>GPAASAGRIERRRARAAVAGRDATGRFTAGQPRRVELDADATSGAFYARYRDGYVSGEPWPGAGPPPPGRVLYGGLGDSRPGLWGAPEAEEARRRFEASGAPAAVWAPELGDAAQQYALITRLLYTPDAEAMGWLQNPRVVPGDVALDQACFRISGAARNSSSFITGSVARAVPHLGYAMAAGRFGWGLAHAAAAVAMSRRYDRAQKGFLLTSLRRAYAPLLARENAALTG[4x];> FTAG

The IE gene product, infected cell protein 4 (ICP4) is a transcriptional regulator with a prominent role within this cascade. ICP4 can induce the expression of E and L genes, while conversely it can act as a repressor notably of itself and also other IE genes. ICP4 homo-dimerization is mediated by the DBD, this region interacts preferentially with a bi-partite and asymmetric DNA consensus sequence RTCGTCnnYnYSG (where R is a purine, Y is a pyrimidine, S is a C or G and n is any base). Here we present the crystal structure of the functionally essential ICP4 DNA binding domain in complex with a segment from its own promoter, revealing a novel homo-dimeric fold.

The combination of the ICP4 DBD, residues 258–487 (ICP4N) with a 19mer DNA duplex matching the consensus site from the ICP4 promoter (IE3_19mer), resulted in the formation of a stoichiometric complex, which can be readily separated by gel filtration. The most complete molecular assembly was present in the ICP4N·IE3_19mer data and comprised protein chains C, D and J with DNA chains G and H which were chosen as the reference ICP4 DBD structure unless stated otherwise. Superposition of chains C and D, which together form a homo-dimer from the same molecular assembly indicated that the individual ICP4N polypeptide chains adopt the same overall fold with a backbone RMSD of 1.15 Å for aa301–484. The crystal structure data indicated that the globular region of the ICP4N homo-dimer contacts the upstream base pairs 1–13 of the IE3_19mer DNA duplex. The IE3_19mer DNA is bound across one edge of the ICP4N dimer interface and the upstream region is partially enveloped by complementary structural features of the protein. The protein residues which contact the DNA are mainly clustered within two regions in both protein chains: first the S-loop (aa411–431) and second the short loop connecting helix α6 to α7, which contains an arginine pair (R456, R457) and therefore we have called aa454–459 the ‘R-turn’. The S-loop forms intermolecular contacts with the R-turn of their dimeric partner; the same loops of different monomers adopt a different conformation depending on their location within the major or minor DNA groove. A dipeptide of F283-T284 (chain J) was also observed in contact with the DNA, notably the aromatic sidechain of F283 intercalates within a kink between base-pairs 14 and 15, where the minor groove width is widened between the bases correspond to YS in the consensus sequence. Therefore these data were indicative of a link between DNA within the YnYSG downstream segment and aa258–289 of ICP4, a predicted IDR. Away from the globular domain, with the exception of a DNA intercalating dipeptide F283 and T284, residues 258–286 were absent from the electron density; this region was shown by solution NMR data to be intrinsically disordered, but involved in DNA binding.> DTLCGSCGGNYTNDEFWICCDVCERWYHGKCVKITPAKAESIKQYKCPSCCT;> ARTKQT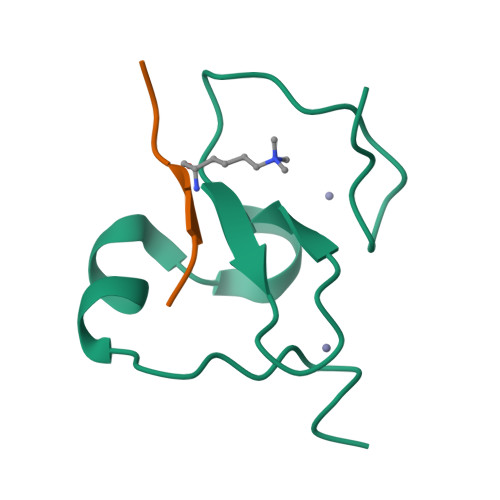A> MTKERFVISRRRTGFGDCLWSLASAWSYAQRTGRTLVIDWRGSCYVEQPFSNAFPAFFEPVEDIAGVPVICDDRVNQLSFPGPFFPRWWNRPSIDCINRPDEQIFRERDELTELFQAREDSEANTIVCDACLMWRCSEEAERLIFRNIKLRSEIRARIDALYEEHFSGHSIIGVHVRHGNGEDIMEHAPYWADSELALHQVCMAIRKA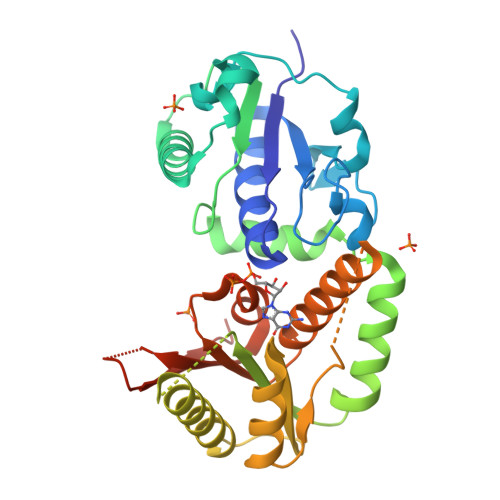KALSYPKPVKVFLCTDSAQVLDQVSGLFPDVFAVPKRFQADRAGPLHSAEMGIEGGASALIDMYLLARCATVIRFPPTSAFTRYARLLVPRIIEFDLSNPGHLTMIDNPYEHFAASHHHHHH> MAEKPKLH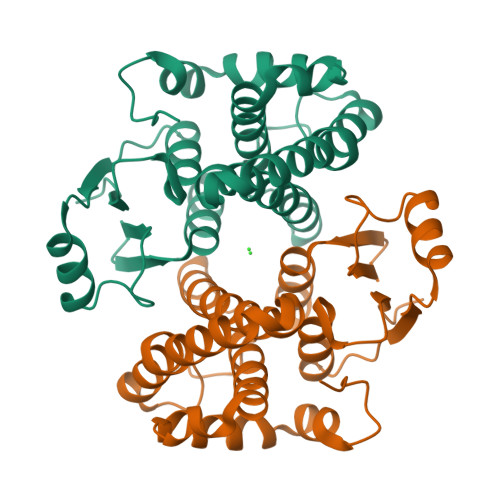YFNARGRMESTRWLLAAAGVEFEEKFIKSAEDLDKLRNDGYLMFQQVPMVEIDGMKLVQTRAILNYIASKYNLYGKDMKERALIDMYSEGILDLTEMIIQLVICPPDQREAKTALAKDRTKNRYLPAFEKVLKSHGQDYLVGNRLTRVDIHLLELLLYVEEFDASLLTSFPLLKAFKSRISSLPNVKKFLQPGSQRKPAMDAKQIEEARKIFRF AMP-activated protein kinase (AMPK) is a metabolic stress-sensing kinase responsible for regulating metabolism in response to energy supply and demand. The AMPK αβγ heterotrimer comprises a catalytic α-subunit associated with β and γ regulatory subunits. Adenine nucleotides (ATP, ADP and AMP) bind interchangeably to the γ subunit where three of the four cystathionine β-synthase (CBS) tandem-repeat sequences provide nucleotide-binding sites1. The α-regulatory subunit-interacting motif 2 (αRIM2)6 is required for sensing the adenine nucleotide bound state of the γ-subunit and transducing this signal to the α-catalytic domain, resulting in either stimulation (AMP) or inhibition (ATP) of AMPK activity.

Secondary structure elements of αRIM2 are crucial for the isoform specificity of C2. We propose the weaker interacting α2 isoform αRIM2 is incompletely engaged upon C2 binding relative to the α1 isoform, resulting in the α-isoform specificity for allosteric and synergistic activation and protection from α-Thr172 dephosphorylation. Importantly the structure reveals density for seven α1 RIM 2 residues, including the main-chain of the nucleotide sensing α-E364 (α2 E368), further supporting our proposal that the α1 RIM2 interacts more strongly with the γ-subunit. Interestingly there was weak density for the carboxyl group of the E364 side-chain, possibly indicating a transient interaction with the γ-subunit residue R70.

>[2x]MGSSHHHHHHHSQDPAEKQKHDGRVKIGHYVLGDTLGVGTFGKVKIGEHQLTGHKVAVKILNRQKIRSLDVVGKIKREIQNLKLFRHPHIIKLYQVISTPTDFFMVMEYVSGGELFDYICKHGRVEEMEARRLFQQILSAVDYCHRHMVVHRDLKPENVLLDAHMNAKIADFGLSNMMSDGEFLRTSCGSPNYAAPEVISGRLYAGPEVDIWSCGVILYALLCGTLPFDDEHVPTLFKKIRGGVFYIPEYLNRSVATLLMHMLQVDPLKRATIKDIREHEWFKQDLPSYLFPEDPSYDANVIDDEAVKEVCEKFECTESEVMNSLYSGDPQDQLAVAYHLIIDNRRIMNQASEFYLASSPPDSFLDDHHLTRPHPERVPFLVAETPRARHTLDELNPQKSKHQGVKKAKWHLGIRSQSKPYDIMAEVYRAMKQLDFEWKVVNAYHLRVRRKNPVTGNYVKMSLQLYLVDNRSYLLDFKSIDDEVVEQRSGSSTPQRSCSAAGLHRPRSSFDSTTAESHSLSGSLTGSLTGSTLSSVSPRLGSHTMDFFEMCASLITTLAR;>MGNTSSERAALERHGGHKTPRRDSSGGTKDGDRPKILMDSPEDADLFHSEEIKAPEKEEFLAWQHDLEVNDKAPAQARPTVFRWTGGGKEVYLSGSFNNWSKLPLTRSHNNFVAILDLPEGEHQYKFFVDGQWTHDPSEPIVTSQLGTVNNIIQVKKTDFEVFDALMVDSQKCSDVSELSSSPPGPYHQEPYVCKPEERFRAPPILPPHLLQVILNKDTGISCDPALLPEPNHVMLNHLYALSIKDGVMVLSATHRYKKKYVTTLLYKPI[2x];>MADLNWETVISSDSSPAVENEHPQETPESNNSVYTSFMKSHRCYDLIPTSSKLVVFDTSLQVKKAFFALVTNGVRAAPLWDSKKQSFVGMLTITDFINILHRYYKSALVQIYELEEHKIETWREVYLQDSFKPLVCISPNASLFDAVSSLIRNKIHRLPVIDPESGNTLYILTHKRILKFLKLFITEFPKPEFMSKSLEELQIGTYANIAMVRTTTPVYVALGIFVQHRVSALPVVDEKGRVVDIYSKFDVINLAAEKTYNNLDVSVTKALQHRSHYFEGVLKCYLHETLETIINRLVEAEVHRLVVVDENDVVKGIVSLSDILQALVLTGGEKKP[2x]> FKPLPISFDDFSDLNRSCFAPGFVFGTASSAFQYEGAAFEDGKGPSIWDTFTHKYPEKIKDRTNGDVAIDEYHRYKEDIGIMKDMNLDAYRFSISWPRVLPKGKLSGGVNREGINYYNNLINEVLANGMQPYVTLFHWDVPQALEDEYRGFLGRNIVDDFRDYAELCFKEFGDRVKHWITLNEPWGVSMNAYAYGTFAPGRCSDWLKLNCTGGDSGREPYLAAHYQLLAHAAAARLYKTKYQASQNGIIGITLVSHWFEPASKEKADVDAAKRGLDFMLGWFMHPLTKGRYPESMRYL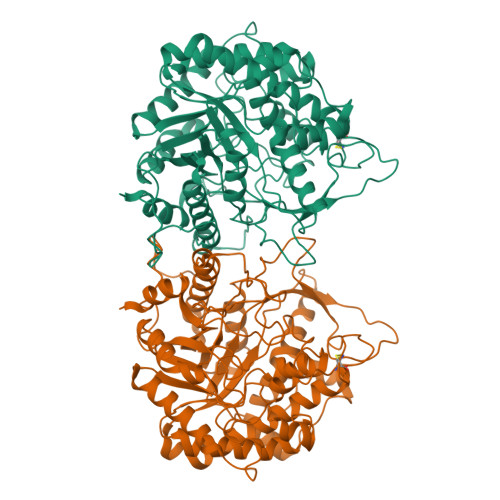VRKRLPKFSTEESKELTGSFDFLGLNYYSSYYAAKAPRIPNARPAIQTDSLINATFEHNGKPLGPMAASSWLCIYPQGIRKLLLYVKNHYNNPVIYITENGRNEFNDPTLSLQESLLDTPRIDYYYRHLYYVLTAIGDGVNVKGYFAWSLFDNMEWDSGYTVRFGLVFVDFKNNLKRHPKLSAHWFKSFLKK Kustd1711 is a putative electron transfer protein encoded on the nitrite oxidoreductase (nxr) gene cluster of anaerobic ammonium-oxidizing (anammox) bacteria and consists of two heme-containing domains and one additional domain. Here, we describe a diheme cytochrome c with high heme redox potentials of about +350 mV, despite having a large overall negative charge, which typically reduces redox potentials. High-resolution crystal structures, spectroelectrochemical measurements, and high-end computational methods show how this is achieved: each heme iron has a calcium cation positioned next to it at a distance of only 6.9 Å, raising their redox potentials by several hundred millivolts through electrostatic interaction. We suggest that this has evolved to provide the protein with a high redox potential despite its large negative surface charge, which it likely requires for interactions with redox partners.

In our 1.75 Å resolution crystal structure, a glycerol molecule from the cryoprotectant binds in between the two hemes. We therefore collected data from a crystal cryoprotected in PEG 1000, which showed that without glycerol, the space between the two hemes is occupied by the side chain of Arg70, but that the structure was otherwise unchanged. As the data from this crystal were of lower quality, we performed all analyses using the 1.75 Å resolution data from the crystal cryoprotected with glycerol. Importantly, in our theoretical calculations of redox potentials (see later), the presence or absence of the glycerol or the Arg70 side chain between the heme groups did not affect the results by more than a few millivolts.

> MNKTMLKIVAFGVAVIGFYMYITVYVTGLSGTGGGGTATGVSAEAGEQIFWGDGQCSTCHKIGSSGSATRGPDQEGLAERAEERAKELGLSSGLEYLVESIIDPEKYVVEGFDKIMPRVYDPPIMLSREKILAVLAYLQSLGGEPDLDAIMKFKDKIPEASKTKVKPWVPPLAVTAEEGEQVFFDESLDVTCGKCHMVNGKGQKVGPELTGIGAIQTPQYFVESILEPSAVIVKGYETVFVITADGIPYNGLIKSDTEEELTLILEESGSVEEVVIPKDEIEDMKKQEVSIMPGNIGELLSVRQFYAVIEYLRSLK7-CHLOROTRYPTOPHAN | 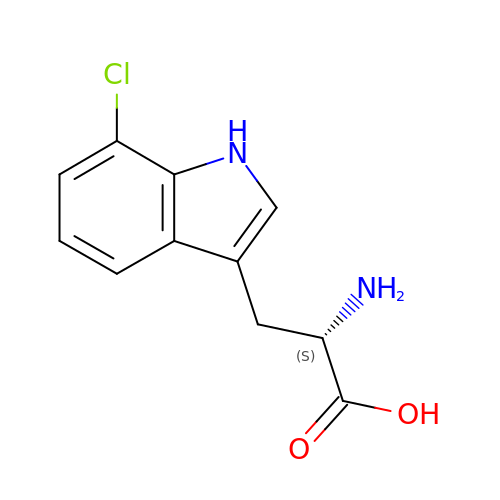C11 H11 Cl N2 O2 | DMQFGLHRDFQKNR-VIFPVBQESA-N Small molecules in the environment can be sensed as attractants or repellents by a repertoire of chemoreceptors termed methyl-accepting chemotaxis proteins (MCPs) or transducer-like proteins (Tlps). Analysis of the crystal structure of the LBDs of C. jejuni Tlp1 and Tlp3 revealed that they have a double Cache (dCache; calcium channels and chemotaxis receptors) fold. dCache domains consist of two tandem subdomains (termed membrane-distal and membrane-proximal) that likely emerged through tandem segmental DNA duplication. We also discovered eight new small-molecule ligands that, in addition to isoleucine, signal through Tlp3 as attractants by binding directly to its LBD, and determined the crystal structures of the respective complexes. The hydrophobic side-chain binding pocket and the conserved protein residues that interact with the ammonium and carboxylate groups of the ligands determine the specificity of this chemoreceptor, which appears to have evolved as a receptor for natural non-polar amino acids.

To identify candidate signal molecules of this class, we generated a virtual library comprising ~2600 L-isoleucine analogues and screened it by docking into the known L-isoleucine binding site of Tlp3 LBD. The three water-soluble compounds with the lowest predicted free energy of binding (4-methyl-L-isoleucine, β-methyl-L-norleucine, and 3-methyl-L-isoleucine) were selected for the subsequent experiments. In the thermal shift assay, the ΔTm values for all three compounds (2.8 °C, 3.7 °C, and 2.0 °C) exceeded the 1.0 °C threshold, suggesting their direct binding to Tlp3 LBD. Among the non-natural amino acids, α-amino-N-valeric acid showed a slightly lower affinity for Tlp3 LBD (168 μM) than isoleucine and leucine, followed by β-methyl-L-norleucine (Kd = 294 μM), 4-methyl-L-isoleucine (Kd = 324 μM), and 3-methyl-L-isoleucine (Kd = 484 μM). Comparison of the crystal structure of Tlp3 LBD/L-isoleucine complex with the final refined structures of Tlp3 LBD in complex with L-leucine, L-valine, α-amino-N-valeric acid, 4-methyl-L-isoleucine, 3-methyl-L-isoleucine, L-alanine, L-phenylalanine, and β-methyl-L-norleucine shows that the binding modes of all the new ligands are very similar to that of isoleucine. The aliphatic side chain of 4-methyl-L-isoleucine forms van der Waals contacts with the side chains of Tyr118, Trp151, and Val171 and is positioned within 4.5 Å of the side chains of Asn116, Val126, Leu128, and Leu144. Furthermore, simultaneous single methyl group substitution at Positions 3 and 4 has a deleterious effect on the binding affinity, as compared to single methyl substitutions at positions 3 or 4: 4-methylisoleucine displays a lower binding affinity (Kd = 324 µM) than L-isoleucine or L-leucine.

>GIDPFTKTSLYESTLKNQTDLLKVTQSTVEDFRSTNQSFTRALEKDIANLPYQSLITEENIINNVGPILKYYRHSINALNVYLGLNNGKVLLSQKSNDAKMPELRDDLDIKTKDWYQEALKTNDIFVTPAYLDTVLKQYVITYSKAIYKDGKIIGVLGVDIPSEDLQNLVAKTPGNTFLFDQKNKIFAATNKELLNPSIDHSPVLNAYKLNGDNNFFSYKLNNEERLGACTKVFAYTACITESADIINKPIYKA[2x]>[2x]VETIELKRGSNSVYVQYDDIMFFESSTKSHRLIAHL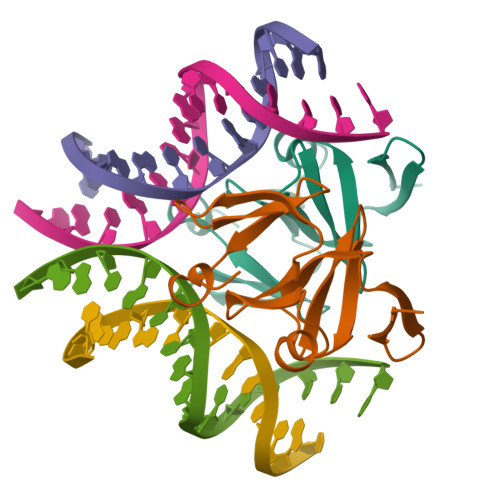DNRQIEFYGNLKELSQLDDRFFRCHNSFVVNRHNIESIDSKERIVYFKNKEHCYASVRNVKKI>MNIVENEICIRTLIDDDFPLMLKWLTDERVLEFYGGRDKKYTLESLKKHYTEPWEDEVFRVIIEYNNVPIGYGQIYKMYDELYTDYHYPKTDEIVYGMDQFIGEPNYWSKGIGTRYIKLIFEFLKKE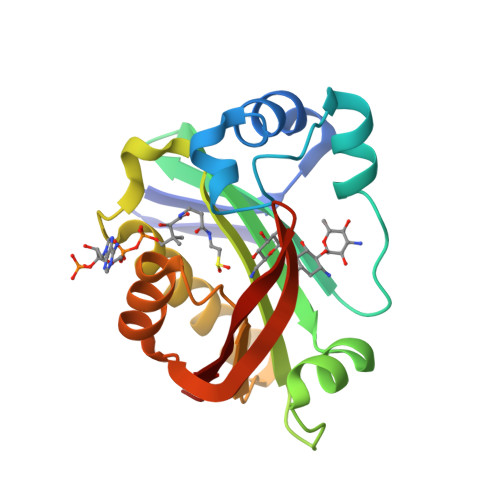RNANAVILDPHKNNPRAIRAYQKSGFRIIEDLPEHELHEGKKEDCYLMEYRY[2x]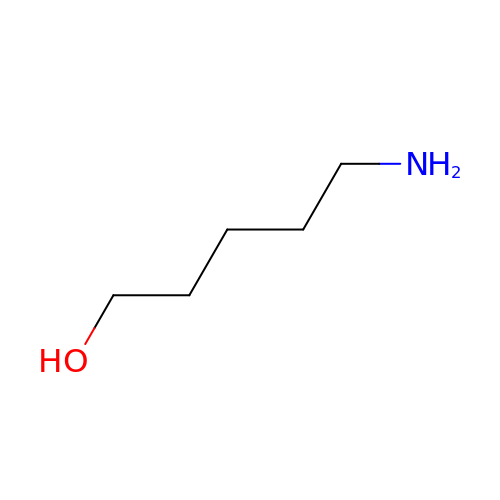5-aminopentan-1-ol | C5 H13 N O | LQGKDMHENBFVRC-UHFFFAOYSA-N>[2x]GSHMASMSEVERALDVLLQEAEELCIGSSVVELDRIPTALEFCREFYSKNQPVVIRKALNWPAIGKWTPKYLIEALGDRS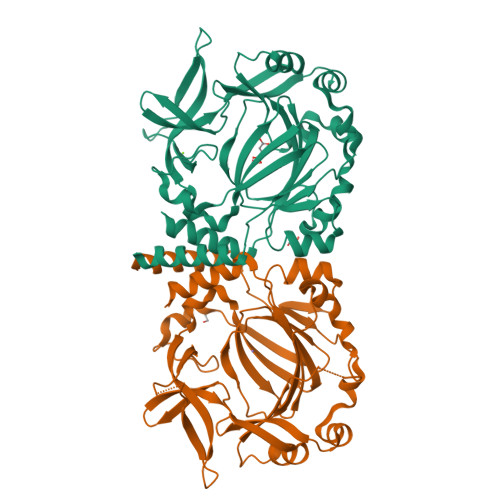VDVAITPNGYADGLATQNGQEYFVLPLETKMKLSEVVRRLDDPTGAVHYIQKQNSNLSVDLPELAADLRVSDLDFAQQSFNKPPDAVNFWLGDERAVTSMHKDPYENVYCVISGHKDFVLIPPHQLSCVPRGIYPTGVYKTSDSGQFYIEPLRDEEGSDQFTEWVSVDPLSPDLAKYPEYARAKPLKVRVHAGDILYLPNYWFHHVSQSHKCIAVNFWYDLDYDSRYCYYRMLEQMTSARSG> MADITETQESLPPFRMGEVGSLGLKVRSGRIYEEPRQALRFPESIKTFQLMMRDPSVAASVNI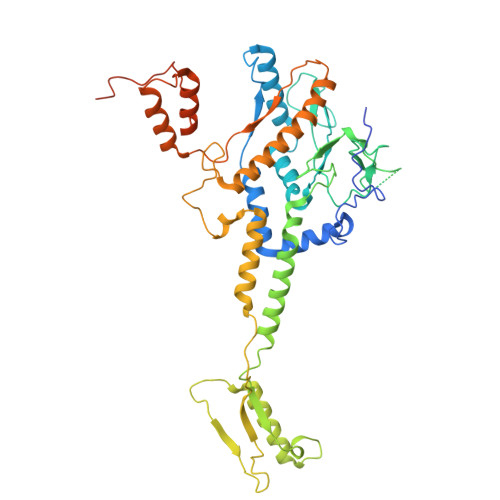IKMFVRKVNWRFVPPKGKEKDAKMIERANFFNSLMNDMEHDWADFINSVMSFCTYGFCVNEKVYKKRQGKKGKYPSKYNDGLIGWAKLPIRNQTTLDKWYFDSDYRKVIGVRQNLRNVSHTAGAINLGEQPLTRKLPRSKFLLFKYDDEYGNPEGRSPLLNAYVPWKYKVQIEEFEAVGVSRDLVGMPKIGLPPDYLGEDAEPEKKAFVKYCQEVVNDLIANDRAGLIWPRFIDPETKEDIFEFSLVSRQGAKAYDTGSIIDRYSKQIMMAFMSDVLAMGQSKYGSFSLADSKTSLLAMSVDILLKQIKNVINRDLVAQTYALNMWDDEEHVEIVYDDIETPDIESIGSYVQKTVAVGAMEVDKALSDKLREHIGLEPADESKPVSENLSPNTQSRSGDGYQTAGEGTAKTPSAKDPSTANKANK>GIDPFTMSPKTVFSTDTHREPIPPQPHPSGARPPQLPRELIPRHVAIVMDGNGRWAKQRGLPRTEGHKAGESSLFDVIEGALELGVPYLSAYAFSTENWKRSPDEVRFLMGFNRDVIRRRRDELHARGVRVRWAGRPGRLWKSVIKELTEAEELTKHNTKLTLQF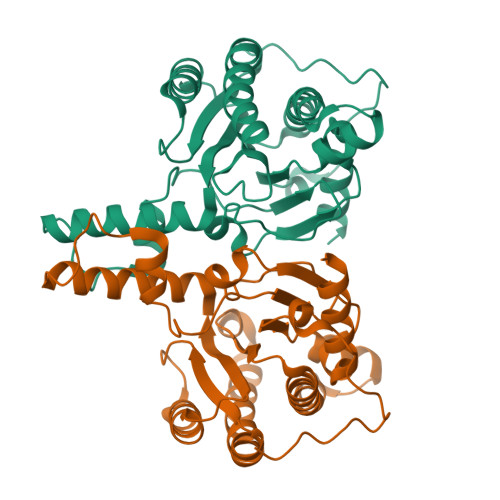CVNYGGRAEIADAAAALARDVAAGRLSPNRVTEATLARYLYHPDIPDVDLFIRSSGEQRLSNFLLWQSSYAEFVFLDTLWPDFDRRHFWQACEIYARRDRRYGGAEPNPVGPPQSAAGAQGQD[6x]> AQYYPGTTKVAQNRRNFCNPEYELEKLREISDEDVVKILGHRAPGEEYPSVHPPLEEMDEPEDAIREMVEPIDGAKAGDRVRYIQFTDSMYFAPAQPYVRSRAYLCRYRGADAGTLSGRQIIETRERDLEKISKELLETEFFDPARSGVRGKSVHGHSLRLDEDGMMFDMLRRQIYNKDTGRVEMVKNQIGDELDEPVDLGEPLDEETLMEKTTIYRVDGE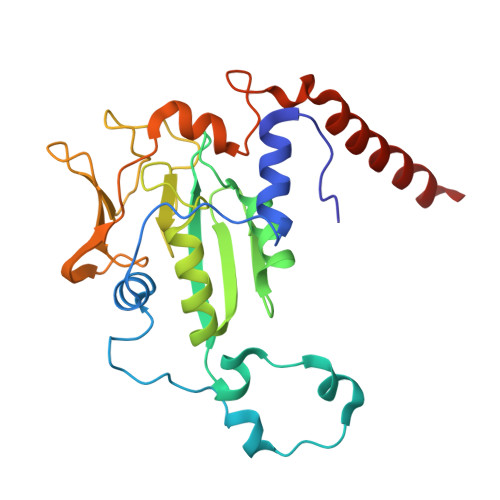AYRDDVEAVEIMQRIHVLRSQGGFNLE> AGCACCTGTA;> ACACCGT;> TCT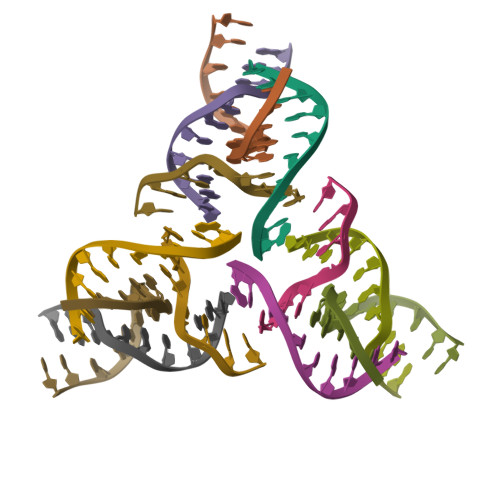GACTGTGGTGC;> CGGACAGTCAG>[2x]TCSTTLIAIAGMT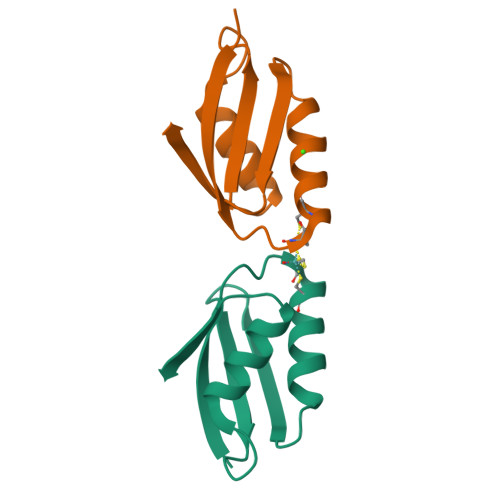CASCVHSIEGMISQLEGVQQISVSLAEGTATVLYNPAVISPEELRAAIEDMGFEASVVS>[4x]MAVDADSANYRIEHDTMGEVRVPAKALWRAQTQRAVENFPISGRGLERTQIRALGLLKGACAQVNSDLGLLAPEKADAIIAAAAEIADGQHDDQFPIDVFQTGSGTSSNMNTNEVIASIAAKGGVTLHPNDDVNMSQSSNDTFPTATHIAATEAAVAHLIPALQQLHDALAAKALDWHTVVKSGRTHLMDAVPVTLGQEFSGYARQIEAGIERVRACLPRLGELAIGGTAV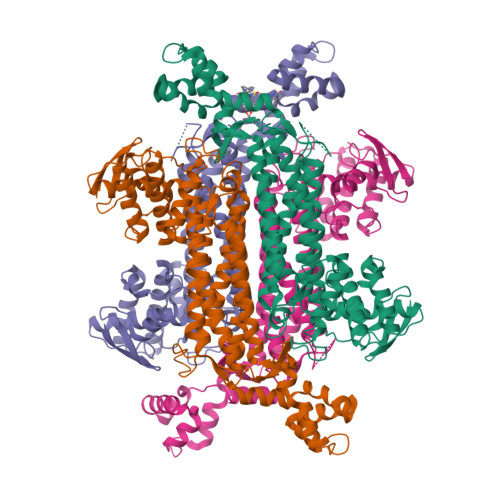GTGLNAPDDFGVRVVAVLVAQTGLSELRTAANSFEAQAARDGLVEASGALRTIAVSLTKIANDIRWMGSGPLTGLAEIQLPDLQPGSSIMPGKVNPVLPEAVTQVAAQVIGNDAAIAWGGANGAFELNVYIPMMARNILESFKLLTNVSRLFAQRCIAGLTANVEHLRRLAESSPSIVTPLNSAIGYEEAAAVAKQALKERKTIRQTVIDRGLIGDRLSIEDLDRRLDVLAMAKAEQLDSDRL> MELKNSISDYTEAEFVQLLKEIEKENVAATDDVLDVLLEHFVKITEHPDGTD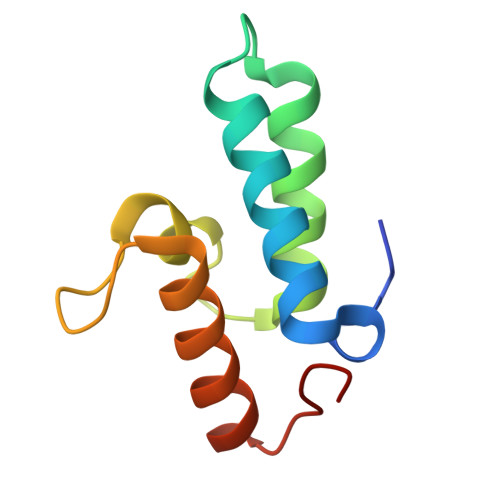LIYYPSDNRDDSPEGIVKEIKEWRAANGKPGFKQG> MGSMAMDTFITRNFQTTIIQKAKNTMAEFSEDPELQPAMLFNICVHLEVC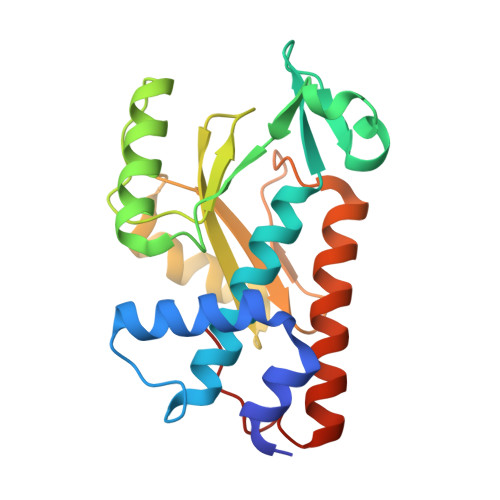YVISDMNFLDEEGKSYTALEGQGKEQNLRPQYEVIEGMPRTIAWMVQRSLAQEHGIETPKYLADLFDYKTKRFIEVGITKGLADDYFWKKKEKLGNSMELMIFSYNQDYSLSNESSLDEEGKGRVLSRLTELQAELSLKNLWQVLIGEEDVE>MMLSATQPLSEKLPAHGCRHVAIIMDGNGRWAKKQGKIRAFGHKAGAKSVRRAVSFAANNGIEALTLYAFSSENWNRPAQEVSALME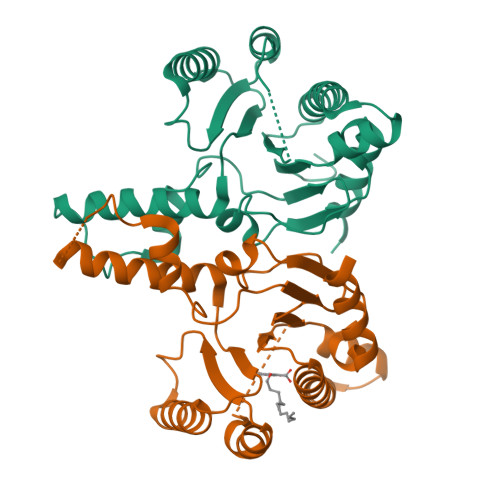LFVWALDSEVKSLHRHNVRLRIIGDTSRFNSRLQERIRKSEALTAGNTGLTLNIAANYGGRWDIVQGVRQLAEKVQQGNLQPDQIDEEMLNQHVCMHELAPVDLVIRTGGEHRISNFLLWQIAYAELYFTDVLWPDFDEQDFEGALNAFANRERRFGGTEPGDETA[2x]>EDPHLRNRPGKGHNYIDGMTQEDATCKPVTYAGACSSFDVLLEKGKFPLFQSYAHHRTLLEAVHDTIIAKADPPSCDLQSAHGNPCMKEKLVMKTHCPNDYQSAHY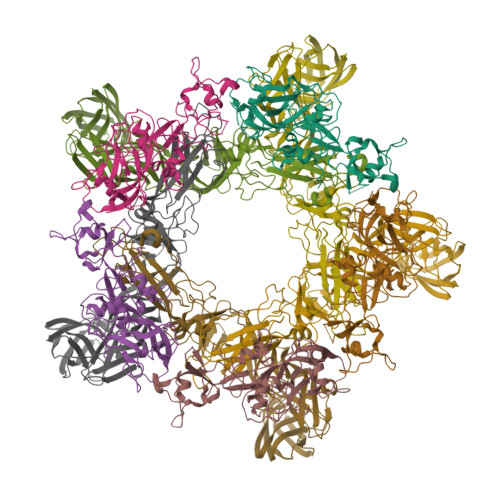LNNDGKMASVKCPPKYELTEDCNFCRQMTGASLKKGSYPLQDLFCQSSEDDGSKLKTKMKGVCEVGVQALKKCDGQLSTAHEVVPFAVFKNSKKVYLDKLDLKTEENLLPDSFVCFEHKGQYKGKLDSGQTKRELKSFDISQCPKIGGHGSKKCTGDAAFCSAYECTAQYANAYCSHANGSGIVQIQVSGVWKKPLCVGYERVVVKRELS[5x];>DPGCSELIQASSRITTCSTEGVNTKCRLSGTALIRAGSVGAEACLMLKGVKEDQTKFLKIKTVSSELSCREGQSYWTGSFSPKCLSSRRCHLVGECHVNRCLSWRDNETSAEFSFVGESTTMRENKCFEQCGGWGCGCFNVNPSCLFVHTYLQSVRKEALRVFNCIDWVHKLTLEITDFDGSVSTIDLGASSSRFTNWGSVSLSLDAEGISGSNSFSFIESPGKGYAIVDEPFSEIPRQGFLGEIRCNSESSVLSAHESCLRAPNLISYKPMIDQLECTTNLIDPFVVFERGSLPQTRNDKTFAASKGNRGVQAFSKGSVQADLTLMFDNFEVDFVGAAVSCDAAFLNLTGCYSCNAGARVCLSITSTGTGSLSAHNKDGSLHIVLPSENGTKDQCQILHFTVPEVEEEFMYSCDGDERPLLVKGTLIAID[5x]> MLRTTHVSWASTAKGYMNRVMVYAHRRRKARYLAPKNAHVRSPLAHKMPEEYGNTWDPRSGVEWHNRM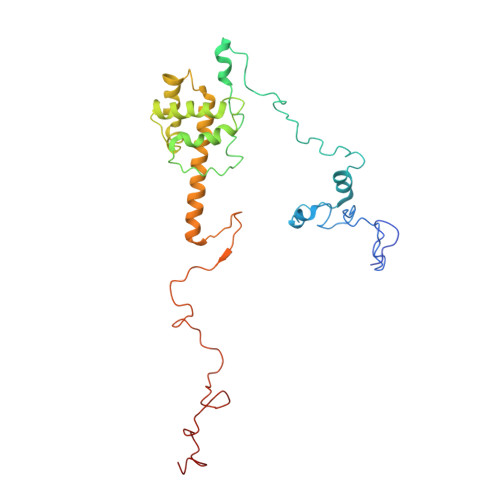RNRNHYRHWPWARWTDDPVRFHQDSVCHRTVSALSTVANNGAPEWDYYAEVGQAYETPSHFPLSYTAPFIYQYTAQCWSREDLQSYLERIEQSSGLRTIADAASRREALYTWWHNAGMNVIPLGVLQHLELVSRDIVAQNARKSYRIEQHERGILRTPEMERYYALPHLRGPSMPVQLAQPSGKYPSGKFTQMMEDVAIHPLQKPDARYKHNMYPA>[2x]SN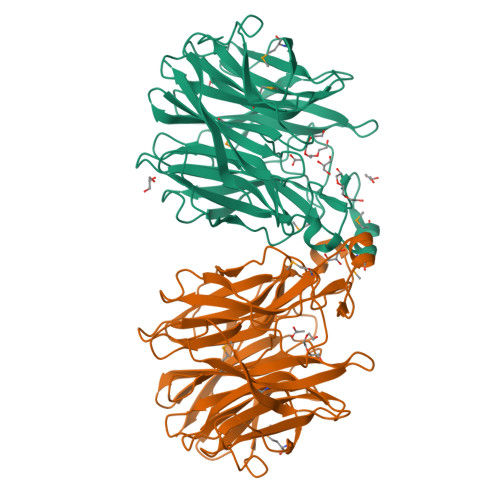AMKLKEISTLLLLFSAMGYRVPARANAGPHLTFTDSIPGVRKVEDVVIYRNEKFHAAFPSVIKKKNGEIVLAFRRAPDRKVFGEKGTNHVDPNSYLVSVKSKDGKTWTPEPELIYSHPFGGSQDPCLLQLKDGTILCASYGWAFLRPDGMENLKKPYFLAGGAVFLGGYVLRSTDGGKSWQGPLYPPHIEPEINYTAMGEKLPAYNRGAMYEGKNGRILWVVAATDRQSPNKTSNHLLISDDKGLTWKYSAPVAVDEKVSFNEASVYETPKGDVVAFLRTAGLGDQACIARSVDGGKTFTAWEKMGFQGHPMHALRLPDNRVLLSYGYRHKPLGIRARILNAECTDFATAPEIVLRTDGGTTDLGYPWAVQLDKNRVLVSYYFNVPGGPQHIAGSILEIR>LSGAVTALILVIASVIIALVVVGFAFGLFGAFTGQGTVAQVGTATLSASTLTLTVTLKNTGASTQVTGVLINGNSGSVSGMTTISAGVNTYTIT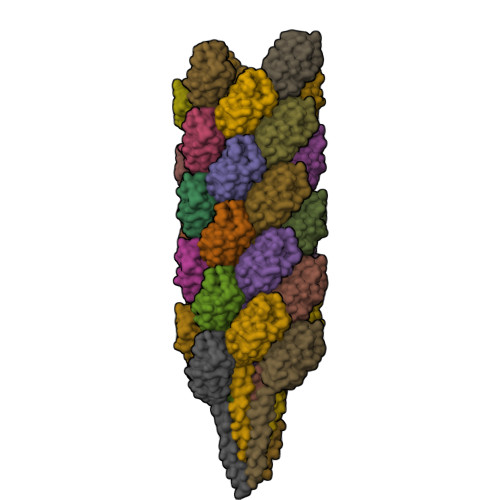ISIGSISTTLRGLVGSTISLTLILSNGETVTVSAIVTS[33x]>[2x]EDICFIAGIGDTNGYGWGIAKELSKRNVKIIFGI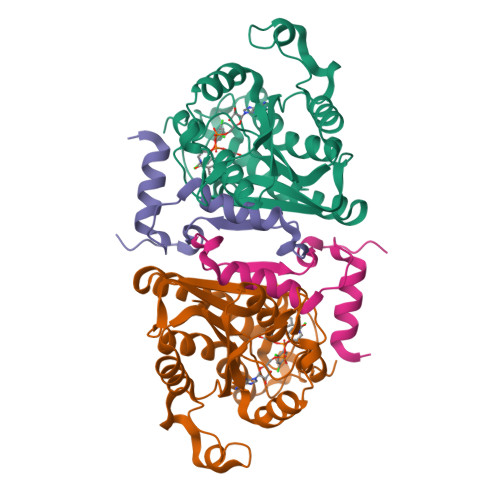WPPVYNIFMKNYKNGKFDNDMIIDKDKKMNILDMLPFDASFDTANDIDEETKNNKRYNMLQNYTIEDVANLIHQKYGKINMLVHSLANAKEVQKDLLNTSRKGYLDALSKSSYSLISLCKYFVNIMKPQSSIISLTYHASQKVVPGYGGGMSSAKAALESDTRVLAYHLGRNYNIRINTISAGPLKSRAATAINK;>YTFIDYAIEYSEKYAPLRQKLLSTDIGSVASFLLSRESRAITGQTIYVDNGLNIMFLPDD[2x]>[2x]XMKQYLELMQKVLDEGTQKNDRTGTGTLSIFGHQMRFNLQDGFPLVTTKRCHLRSIIHELLWFLQGDTNIAYLHENNVTIWDEWADENGDLGPVYGKQWRAWPTPDGRHIDQITTVLNQLKNDPDSRRIIVSAWNVGELDKMALAPCHAFFQFYVADGKLSCQLYQRSCDVFLGLPFNIASYALLVHMMAQQCDLEVGDFVWTGGDTHLYSN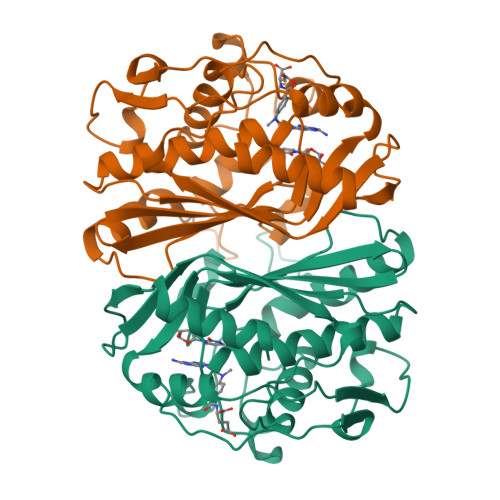HMDQTHLQLSREPRPLPKLIIKRKPESIFDYRFEDFEIEGYDPHPGIKAPVAI> MRARRSPAINTLDAQLQQADASPASAPSPSSPSSAPLAPSDLDDVLCRHTLRLPKPASTGQEAALRLLSRFNGALPSLRGQTILAKVLSVDSERVT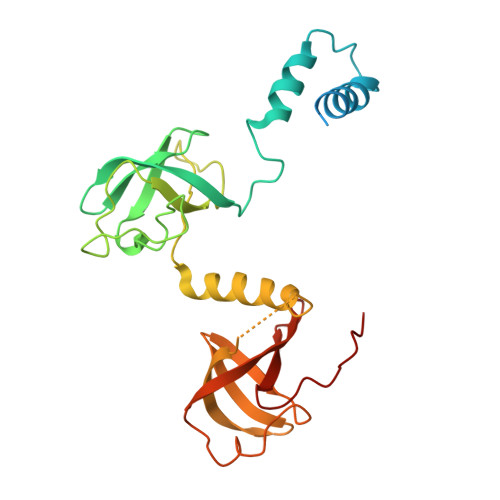VDTGYNGVAEVPRADVSIAHVHTADGAAPVRPTTSDVRPGDLLRLRVDAPYTPYGDMQLTAVREESEFKRRLAWGELRRAMEAGQPVSGRVLNDCVGGFAVGVAGFVAFLPSAMAARDTTQRVGSLQSFRIVAMDEARRRITLRDAGVAAAGFRRVG>[2x]MAHMERFQKVYEEVQEFLLGDAEKRFEMDVHRKGYLKSMMDTTCLGGKYNRGLCVVDVAEAMAKDTQMDAAAMERVLHDACVCGWMIEMLQAHFLVEDDIMDHSKTRRGKPCWYLHPGVTAQVAINDGLILLAWATQMALHYFADRPFLAEVLRVF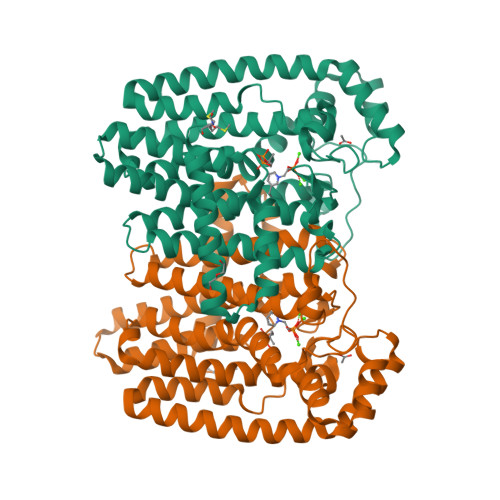HDVDLTTYIGQLYDVTSMVDSAKLDAKVAHANTTDYVEYTPFNHRRIVVYKTAYYTYWLPLVMGLLVSGTLEKVDKKATHKVAMVMGEYFQVQDDVMDCFTPPEKLGKIGTDIEDAKCSWLAVTFLTTAPAEKVAEFKANYGSTDPAAVAVIKQLYTEQNLLARFEEYEKAVVAEVEQLIAALEAQNAAFAASVKVLWSKTYKRQK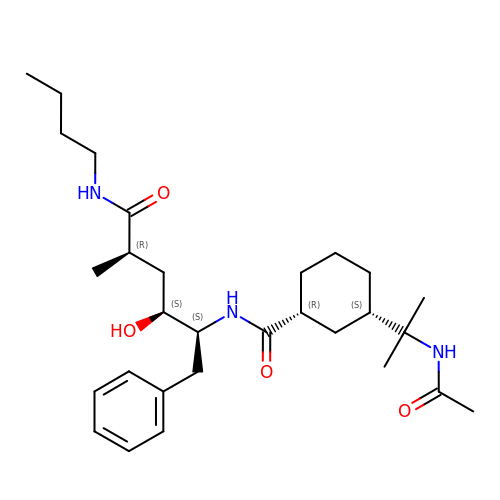(1R,3S)-3-[1-(acetylamino)-1-methylethyl]-N-[(1S,2S,4R)-1-benzyl-5-(butylamino)-2-hydroxy-4-methyl-5-oxopentyl]cyclohexanecarboxamide | C29 H47 N3 O4 | NGUMIHCAWWHVPZ-MTKOPPBXSA-N> MSLTRRDFVKLCTGTVAGFGISQMF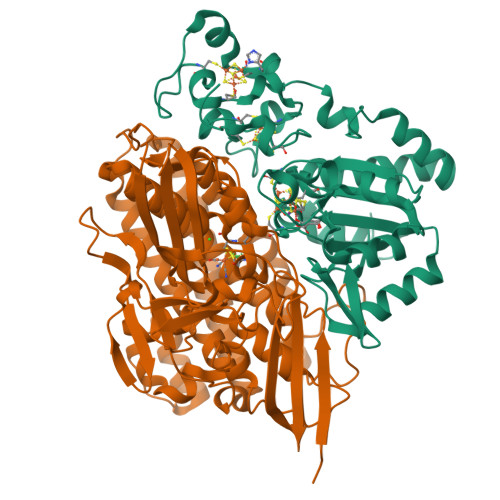HPAVHEALAGTLTGERPPVFWLQGQGCTGCSVTLLNSVHPSIADVLLKVISLEFHPTVMAWEGEHAIEHMRKVAEKFKGKFFLVIEGSVPVEADGKYCIIGEANHHEISMVDALKEFGPNAAAVLAVGTCAAYGGIPAAEGSETGATAVSKFLGDNGIKTPVVNIPGCPPHPDWIVGTVVLALDAIKKNGLEGGLAEVVKVLDSDGRPTPFFGRNIHENCPYLDKYDEGVMSATFTDKVGCRYDLGCKGPMTMADCFERKWNGGVNWCVQNAVCIGCVEPDFPDGKSPFYQA;> WSHPQFEKGATGRTTIAIDPVTRIEGHLKAEVVVENGKVVDARLSGGMYRGFETILRGRDPRDASQIVQRICGVCPTAHSTASVLALDEAFGAKVPNNGRITRNLIFGANYLQSHILHFYHLSAQDFVQGPDTAPFVPRFPKSDLRLSKELNKAGVDQYIEALEVRRICHEMVALFGGRMPHVQGQVVGGATEIPTKEKLVEYAARFKKVRDFVEQKYVPVVYTIGSKYKDMFKVGQGFKAALCVGAFPLDNSGKKHLFMPGVYAKGKDMPFDPSKIKEYVKYSWFAEETTGLNYKEGKTIPAPDKAGAYSFVKAPRYDGLSLEVGPLARMWVNNPELSPVGKKLLKDLFGISAKKFRDLGEEAAFSLMGRHVARAEETYYMLGAIEGWLKEIKAGEDTVVMPAVPASAEGTGFTEAPRGSLLHYVKVKDSKIDNYQIVSASLWNCNPRDDMGQRGAVEEALIGIPVDDIQNPVNVARLIRAFDPULGCAVHVLHAESGKVAVIEVK> GSNQKAVILDEQAIRRALTRIAHEMIERNKGMNNCILVGIKTRGIYLAKRLAERIEQIEGNPVTVGEIDITLYRDDLSKKTSNDEP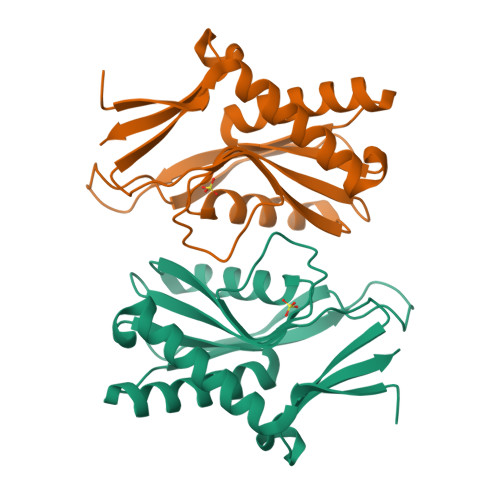LVKGADIPVDITDQKVILVDDVLYTGRTVRAGMDALVDVGRPSSIQLAVLVDRGHRELPIRADYIGKNIPTSKSEKVMVQLDEVDQNDLVAIYENEK>[6x]SLEIPSKQIDYRDVFIEFLTTFKGNNNQNKYIERINELVAYRKKSLIIEFSDVLSFNENLAYEIINNTKIILPILEGALYDHILQLDPTYQRDIEKVHVRIVGIPRVIELRKIRSTDIGKLITIDGILVKVTPVKERIYKATYKHIHPDCMQEFEWPEDEEMPEVLEMPTICPKCGKPGQFRLIPEKTKLIDWQKAVIQERPEEVPSGQLPRQLEIILEDDLVDSARPGDRVKVTGILDIKQDSPVKRGSRAVFDIYMKVSSIEVSGGSGGSSEEDEKKIKDLAKDPWIRDRIISSIAPSIYGHWELKEALALALFGGVPKVLEDTRIRGDIHILIIGDPGTAKSQMLQFISRVAPRAVYTTGKGSTAAGLTAAVVREKGTGEYYLEAGA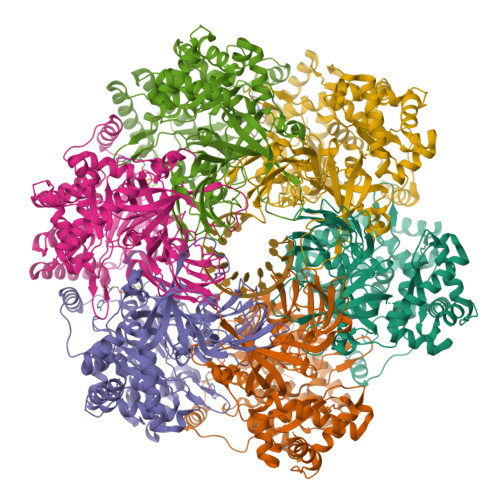LVLADGGIAVIDEIDKMRDEDRVAIHEAMEQQTVSIAKAGIVAKLNARAAVIAAGNPKFGRYISERPVSDNINLPPTILSRFDLIFILKDQPGEQDRELANYILDVHSGKSTKNIIDIDTLRKYIAYARKYVTPKITSEAKNLITDFFVEMRKKSSETPDSPILITPRQLEALIRISEAYAKMALKAEVTREDAERAINIMRLFLESVGVDMESGKIDID> VVGATDTS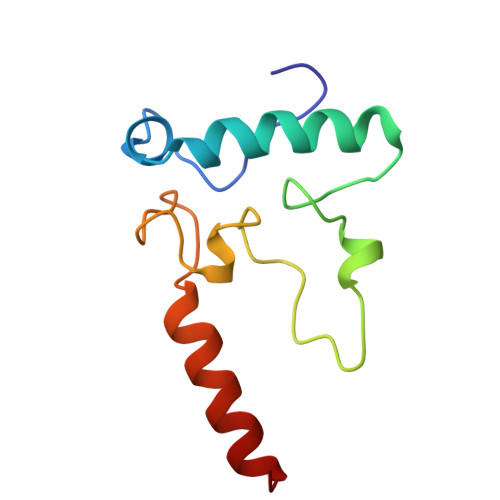TGTLDVANVTDPSTLALLATGAVMINRASGQNDGLVSRCSSLFGQVISTSYHWNHLDEINQLLGVRGANAEDPVAVIRTHVNRLKLQGV> MGGSHHHHHHGMASLAPGSSRVELFKRKNSTVPFEESNGTIRERVVHSFRIPTIVNVDGVMVAIADARYETSFDNSFIETAVKYSVDDGATWNTQIAIKNSRASSVSRVMDATVIVKGNKLYILVGSFNKTRNSWTQHRDGSDWEPLLVVGEVTKSAANGKTTATISWGKPVSLKPLFPAEFDGILTKEFIGGVGAAIVASNGNLVYPVQIADMGGRVFTKIMYSEDDGNTWKFAEGRSKFGCSEPAVLEWEGKLIINNRVDGNRRLVYESSDMGKTWVEALGTLSHVWTNSPTSNQQDCQSSFVAVTIEGKRVMLFTHPLNLKGRWMRDRLHLWMTDNQRIFDVGQISIGDENSGYSSVLYKDDKLYSLHEINTNDVYSLVFVRLIGELQLMKSVVRTWKEEDNHLASICTPVVPATPPSKGGCGAAVPTAGLVGFLSHSANGSVWEDVYRCVDANVANAERVPNGLKFNGVGGGAVWPVARQGQTRRYQFANYRFTLVATVTIDELPKGTSPLLGAGLEGPGDAKLLGLSYDKNRQWRPLYGA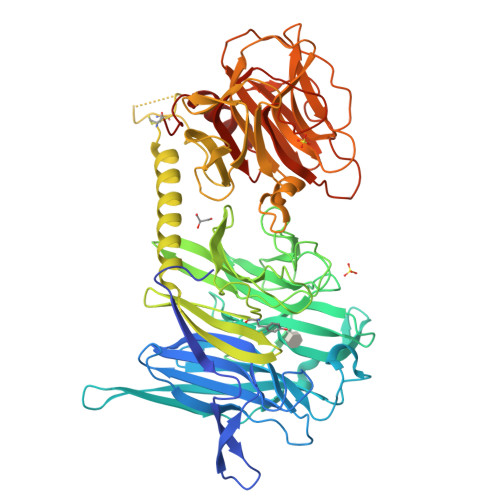APASPTGSWELHKKYHVVLTMADRQGSVYVDGQPLAGSGNTVVRGATLPDISHFYIGGPRSKGAPTDSRVTVTNVVLYNRRLNSSEIRTLFLSQDMIGTDGGAGTAA>RKRLKSSCKRHPLYVDFSDVGWNDWIVAPPGYHAFYCHGECPFPLADHLNSTNHAIVQTLVNSVNSKIPKACCVPTELSAISMLYLDENEKVVLKNYQDMV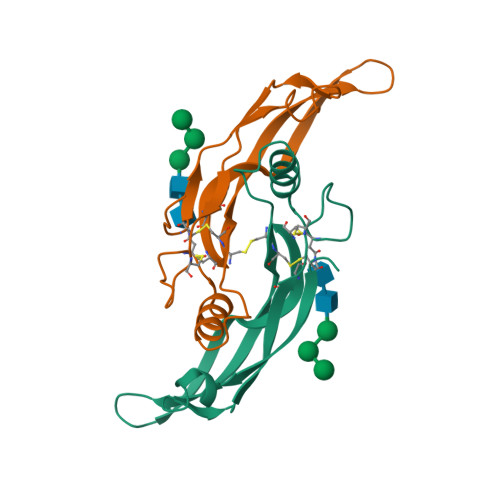VEGCGCR[4x]>PALRMITHISPLGSMDMLSQLEVDMLKRTASSDLYQLFRNCSLAVLNSGSLTDNSKELLSRFENFDINVLRRERGVKLELINPPEEAFVDGRIIRALQANLFAVLRDILFVYGQIHNTVRFPNLNLDNSVHITNLVFSILRNARALHVGEAPNMVVCWGGHSINENEYLYARRVGNQLGLRELNICTGCGPGAMEAPMKGAAVGHAQQRYKDSRFIGMTEPSIIAAEPPNPLVNELIIMPDIEKRLEAFVRIAHGIIIFPGGVGTAEALLYLLGILMNPANKDQVLPLIL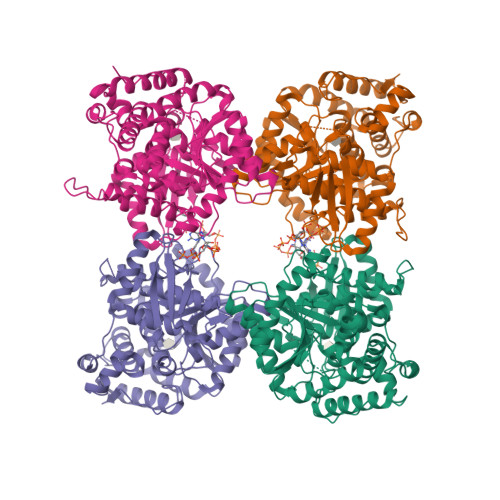TGPKESADYFRVLDEFVVHTLGENARRHYRIIIDDAAEVARQMKKSMPLVKENRRDTGDAYSFNWSMRIAPDLQMPFEPSHENMANLKLYPDQPVEVLAADLRRAFSGIVAGNVKEVGIRAIEEFGPYKINGDKEIMRRMDDLLQGFVAQHRMKLPGSAYIPCYEICT[4x]>GHMSKPSYKVADISLAEWGRKAIIIAENEMPGLMACRKKYGPSKPLKGARITGCLHMTVQTAVLIETLVELGAQVQWSSCNIFSTQDNAAAAIAATGVPVYAWKGETDEEYMWCIEQTLVFPDGQPLNMILDDGGDLTNLVHEKFPQYLKNIKGLSEETTTGVHNLYKMFKEGRLGVPAINVNDSVTKSKFDNLYGCRESLIDGIKRATDVMIAGKVCCVAGYGDVGKGCAQALKGFGGRVIVTEVDPINALQAAMEGYEVTTMEEASKEASIFVTTTGCRDIITSVHLQQMPDDAIVCNIGHFDIEIDVDWLNANAKEKVNVKPQVDRYTMQSGKHIILLA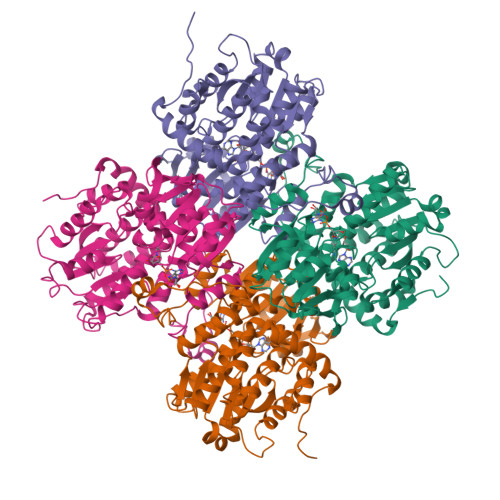EGRLVNLGCAHGHPSFVMSNSFTNQVLAQIELWTKSDKYAVGVHVLPKILDEEVASLHLEKLGVKLTKLTEKQATYLGVSQTGPFKPDHYRY[4x]Poxviruses are unique in requiring eleven transmembrane proteins that form the entry fusion complex (EFC). The fusion apparatus is embedded in the MV membrane and consists of eleven proteins namely A1610, A2111, A2812, F913, G314, G915, H216, J517, L118, L519, and O320, which comprise the entry fusion complex (EFC). F9, the subject of this study, is a 23.8 kDa protein with a putative transmembrane domain near the C-terminus. Here, we report the 2.10 Å structure of F9 and demonstrate a fold similar to L1 but without a hydrophobic cavity.

The VACV strain Western Reserve F9 ectodomain, consisting of residues 1–176 with an added N-terminal 6-histidine tag, was refolded from bacterially-produced inclusion bodies and purified to near homogeneity by immobilized metal affinity chromatography (IMAC) and size exclusion chromatography (SEC). F9 crystallized with four molecules in the asymmetric unit of the crystal used for data collection for refinement, resulting in the 2.10 Å structure. The F9 ectodomain exhibits a bundle of five α-helices (α) packed against two pairs of β-sheets (β). Between α3 and α4, a loop of 12 amino acids protrudes starting with Gly90 and ending with Ser101. As the transmembrane domain begins after the α5 helix, both ends of F9 are close to each other and to the viral membrane. The atomic structure revealed that Cys33 and Cys55, Cys47 and Cys127, and Cys107 and Cys149 form three pairs of disulfide bonds. Cys47 is located in β2 and together with Cys127 it forms a disulfide bond, which stabilizes the β-sheet pairs at the bottom of the molecule. In F9, α3 turns proximal whereas in L1 α3 is located sideward forming the entrance into the hydrophobic cavity. This cavity is missing in F9, although a hydrophobic area similar to L1 is found. With regard to the divergence of F9, its differing orientation of helix α3, its absence of a myristoylation site, and its lack of a hydrophobic cavity likely contribute to F9 functional differences from L1.

>[4x]MAETKEFKTLYNLFIDSYLQKLAQHSIPTNVTCAIHIGEVIGQFKNCALRITNKCMSNSRLSFTLMVESFIEVISLLPEKDRRAIAEEIGIDLDDVPSAVSKLEKNCNAYAEVNNIIDIQKLDIGECSAPPGQHMLLQIVNTGSAEANCGLQTIVKSLNKIYVPPIIENRLPYYDP9-(3-DEOXY-BETA-D-RIBOFURANOSYL)GUANINE | C10 H13 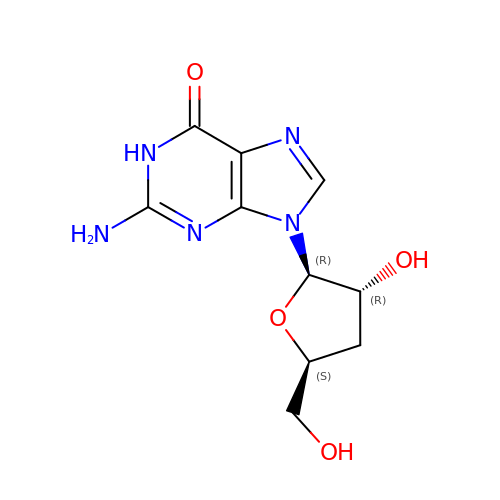N5 O4 | OROIAVZITJBGSM-OBXARNEKSA-N>MDAQYDISFADVEKAHLNIQDSVHLTPVLTSSILNQIAGRNLFFKCELFQKTGSFKIRG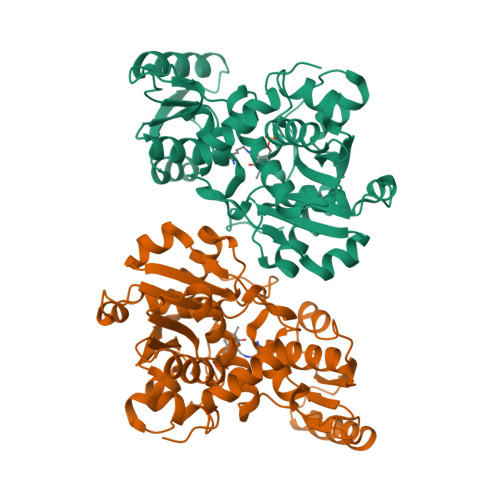ALNAIRGLIPDTLEGKPKAVVTHSSGNHGQALTYAAKLEGIPAYIVVPQTAPNCKKLAIQAYGASIVYSEPSDESRENVAQRIIQETEGILVHPNQEPAVIAGQGTIALEVLNQVPLVDALVVPVGGGGMVAGIAITIKTLKPSVKVYAAEPSNADDCYQSKLKGELTPNLHPPETIADGVKSSIGLNTWPIIRDLVDDVFTVTEDEIKYATQLVWERMKLLIEPTAGVGLAAVLSQHFQTVSPEVKNICIVLSGGNVDLTSLSWVKQAERPAPHHHHHH[2x]> GPLGSGKKCYKLENEKLFEEFLELCKMQTADHPEVVPFLYNRQQRA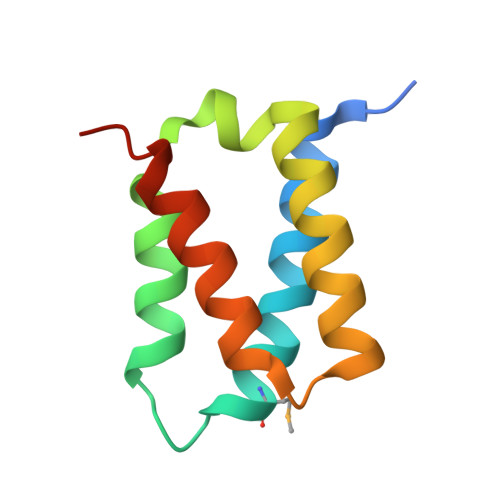HSLFLASAEFCNILSRVLSRARSRPAKLYVYINELCTVLKAHSAKKKLN>[4x]KGTFKDYVRDRADLNKDKPVIPAAALAG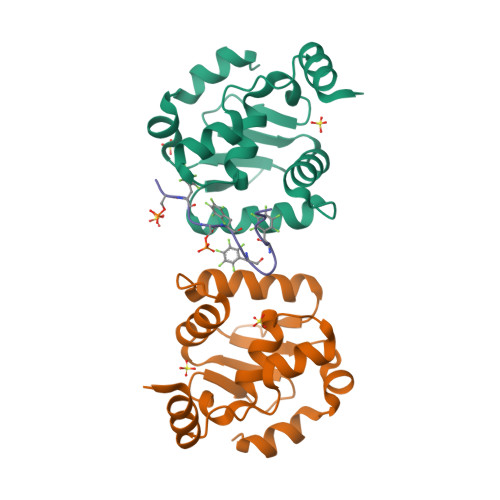YTGSGPIQLWQFLLELLTDKSCQSFISWTGDGWEFKLSDPDEVARRWGKRKNKPKMNYEKLSRGLRYYYDKNIIHKTAGKRYVYRFVCDLQSLLGYTPEELHAMLDVKPDAD;>PSFDSFDFEDFPAALWX[2x]> MH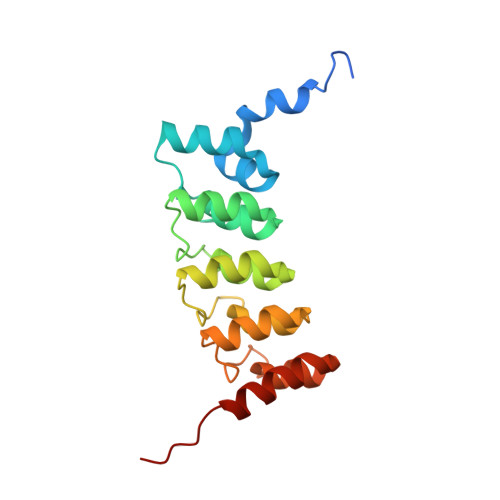HHHHHSSGRENLYFQGSTTPLLANSLSVHQLAAQGEMLYLATRIEQENVINHTDEEGFTPLMWAAAHGQIAVVEFLLQNGADPQLLGKGRESALSLACSKGYTDIVKMLLDCGVDVNEYDWNGGTPLLYAVHGNHVKCVKMLLESGADPTIETDSGYNSMDLAVALGYRSVQQVIESHLLKLLQNIKE> MGRILDISGQPFDFDDEMQSRSDELAMVMKRTQEHPSSGVTPNRAAQMLRDAERGDLTAQADLAFDMEEKDTHLFSELSKRRLAIQALEWRIAPARDASAQEKKDADMLNEYLHDAAWFEDALFDAGDAILKGYSMQEIEWGWLGKMRVPVALHHR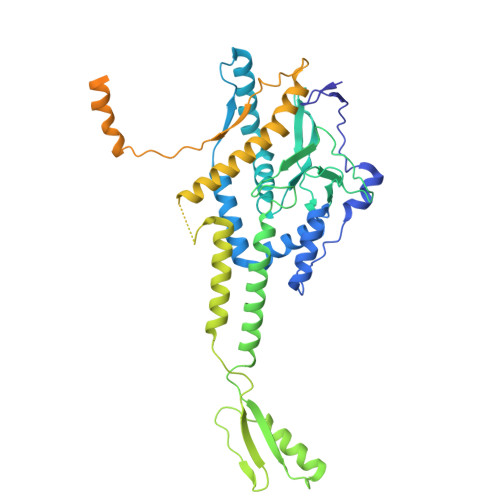DPALFCANPDNLNELRLRDASYHGLELQPFGWFMHRAKSRTGYVGTNGLVRTLIWPFIFKNYSVRDFAEFLEIYGLPMRVGKYPTGSTNREKATLMQAVMDIGRRAGGIIPMGMTLDFQSAADGQSDPFMAMIGWAEKAISKAILGGTLTTEAGDKGARSLGEVHDEVRREIRNADVGQLARSINRDLIYPLLALNSDSTIDINRLPGIVFDTSEAGDITALSDAIPKLAAGMRIPVSWIQEKLHIPQPVGDEAVFTIQPVVPDNGSQKEAALSAEDIPQEDDIDRMGVSPEDWQRSVDPLLKPVIFSVLKDGPEAAMNKAASLYPQMDDAELIDMLTRAIFVADIWGRLDAAADH>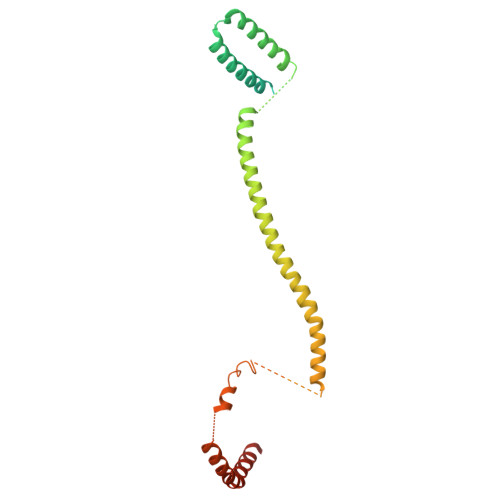 MSGKANASKKNAQQLKRNPKRKKDNEEVVLSENKVRNTVKKNKNHLKDLSSEGQTKHTNLKHGKTAASKRKTWQPLSKSTRDHLQTMMESVIMTILSNSIKEKEEIQYHLNFLKKRLLQQCETLKVPPKKMEDLTNVSSLLNMERARDKANEEGLALLQEEIDKMVETTELMTGNIQSLKNKIQILASEVEEEEERVKQMHQINSSGVLSLPELSQKTLKAPTLQKEILALIPNQNALLKDLDILHNSSQMKSMSTFIEEAYKKLDASHHHHHH> STGPVAPLPTPPNFPNDIALFQQ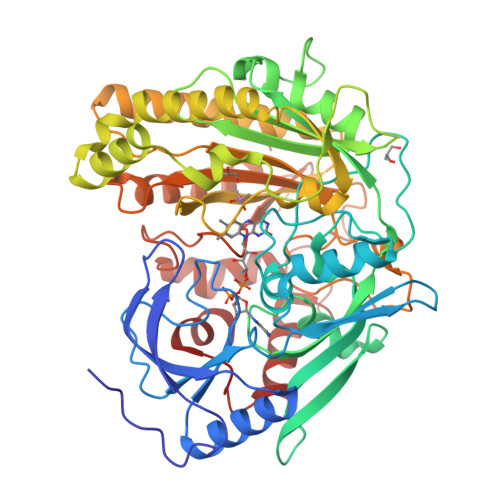AYQNWSKEIMLDATWVCSPKTPQDVVRLANWAHEHDYKIRPRGAMAGWTPLTVEKGANVEKVILADTMTHLNGITVNTGGPVATVTAGAGASIEAIVTELQKHDLGWANLPAPGVLSIGGALAVNAHGAALPAVGQTTLPGHTYGSLSNLVTELTAVVWNGTTYALETYQRNDPRITPLLTNLGRCFLTSVTMQAGPNFRQRCQSYTDIPWRELFAPKGADGRTFEKFVAESGGAEAIWYPFTEKPWMKVWTVSPTKPDSSNEVGSLGSAGSLVGKPPQAREVSGPYNYIFSDNLPEPITDMIGAINAGNPGIAPLFGPAMYEITKLGLAATNANDIWGWSKDVQFYIKATTLRLTEGGGAVVTSRANIATVINDFTEWFHERIEFYRAKGEFPLNGPVEIRCCGLDQAADVKVPSVGPPTISATRPRPDHPDWDVAIWLNVLGVPGTPGMFEFYREMEQWMRSHYNNDDATFRPEWSKGWAFGPDPYTDNDIVTNKMRATYIEGVPTTENWDTARARYNQIDPHRVFTNGFMDKLLP>MSLTMVSEVQPVSPASLDAPLENAVEIIETVISSLHQGDAPLVGQTDSGKIWMFRYGSAEVFVQLSGHTEE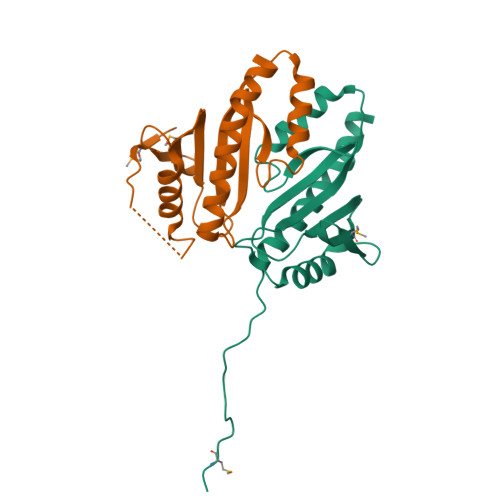DFLTIWSPVLPLPVADELALYRKLLTLNWLTTFEAHFAIAEEQVQVVASRTLGGITAGEISRLITIVATLADDYDDALRAEFKGEGHHHHHH[2x]2-amino-2-deoxy-beta-D-glucopyranose | C6 H13 N O5 | 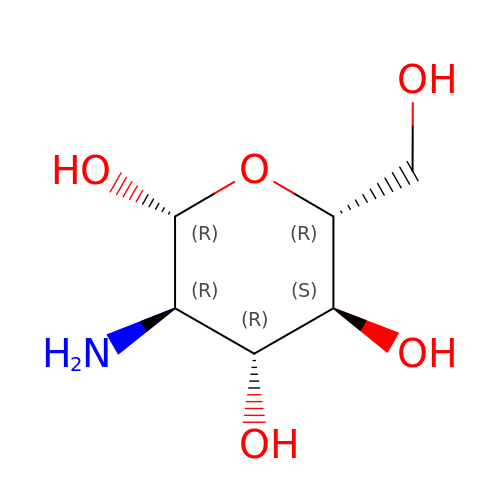MSWZFWKMSRAUBD-QZABAPFNSA-N Two main phospholipase A2 (PLA2) subclasses are often found in bothropic venoms: catalytic PLA2s and the myotoxic PLA2-like toxins. PLA2-like proteins are catalytically inactive proteins due to some natural amino acid substitutions, including Asp49Lys and Tyr28Asn, leading to Ca+2 coordination inability. Some of these regions comprise the myotoxic site (Lys20, Lys115 and Arg118) — subsequently called the membrane docking site (MDoS) — and the membrane disruption site (MDiS) composed of the conserved residues Leu121 and Phe12533. In this work, we studied the binding behaviour between MjTX-I, a myotoxic PLA2s-like isolated from Bothrops moojeni venom, and the suramin molecule using a broad combination of techniques, including myographic assays, molecular dynamic simulations, dynamic light scattering (DLS), small angle X-ray scattering (SAXS), isothermal titration calorimetry (ITC) and X-ray crystallography.

The MjTX-I/suramin crystal structure displays two toxin protomers that interact through one suramin molecule, leading to a PLA2-like compact dimeric assembly formation. According to the crystallographic structure, suramin binds to both protomers of the MjTX-I homodimeric structure making different contacts in each protomer, so we considered the binding events as non-identical. Comparison of the monomers of native MjTX-I and the monomers of the toxin complexed with suramin yielded an average RMSD lower than 0.8 Å, revealing that ligand binding did not affect the tertiary structure of the protein. While the native MjTX-I crystal structure is composed of two dimers in an “extended assembly” that gives rise to a tetrameric array, the MjTX-I/suramin complex presents a dimeric “compact assembly”. However, a deeper analysis showed that there are important distortions in the residue configurations that compose the MDiS region. The distances between Cβ from the residues (Leu122 and Phe125) were between 8–9 Å for both monomers. Thus, according to this classification, both monomers of MjTX-I/suramin are in the non-canonical conformation and are thus unable to interact with membranes. The first one is related to the natural substitution Arg118Asp from the MDoS region of the MjTX-I. The second is related to the binding of the suramin molecule that hides several basic residues, particularly Arg34, Lys49, Lys53, Lys69, and Lys70, which are related to the putative-MDoS suggested in the previous section. Thus, MjTX-I inhibition by the suramin may be related to two causes: (i) distortion of MDiS from both monomers impairing the membrane disruption mechanism by the toxin; and (ii) surface electrostatic changes of the complex that interfere with the toxin membrane dockage process (putative-MDoS is partially hidden).

>[2x]SLVELGKMILQETGKNPVKSYGAYGCNCGVLGRGKPKDATDRCCYVHKCCYKKLTNCNPKKDRYSYDWKNKTIVCGEENPCLKQLCECDKAVAICLRENKGTYNKKRDVYLKPFCDKGRDC>[2x]DSYYQRSDWTADEEQILL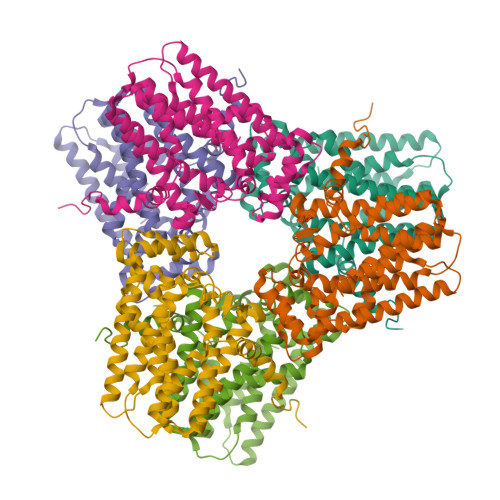GPFDYLESLPGKNMRSQLIQSFNTWLKVPTESLDVIIKVISMLHTAYLLIDDIQDQSILRRGQPVAHSIFGTAQAMNSGNYVYFLALREVQKLQNPKAISIYVDSLIDLHRGQGMELFWRDSLMCPTEEQYLDMVANKTGGLFCLAIQLMQAEATIQVDFIPLVRLLGIIFQICDDYLNLKSTAYTDNKGLCEDLTEGKFSFPIIHSIRSNPGNRQLINILKQKPREDDIKRYALSYMESTNSFEYTRGVVRKLKTEAIDTIQGLEKHGLEENIGIRKILARMSLEL> MSLTGRAFAIPLRTRFRGITVREGMLVRGAAGWGEFSPFAEYGPRECARWWAACYEAAELGWPAPVRDTVPVNATVPAVGPEEAARIVASSGCTTAKVKVAERGQSEANDVARVEAVRDALGPRGRVRIDVNGAWDVDTAVRMIRLLDRFELEYVEQPCATVDELAEVRRRVSVPI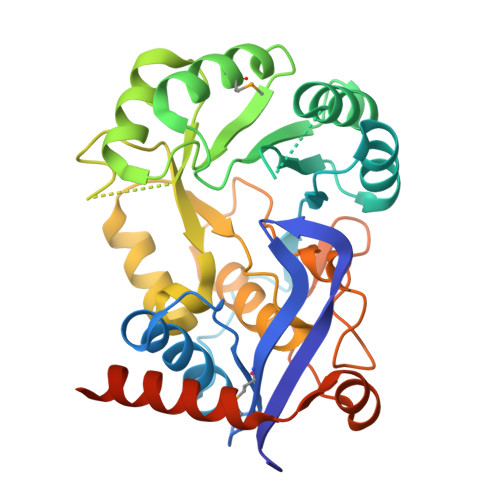AADESIRRAEDPLRVRDAEAADVVVLKVQPLGGVRAALRLAEECGLPVVVSSAVETSVGLAAGVALAAALPELPYACGLATLRLLHADVCDDPLLPVHGVLPVRRVDVSEQRLAEVEIDPAAWQARLAAARAAWEQVEREPGPEGHHHHHH>GAMAKGAVTKLKFNSPI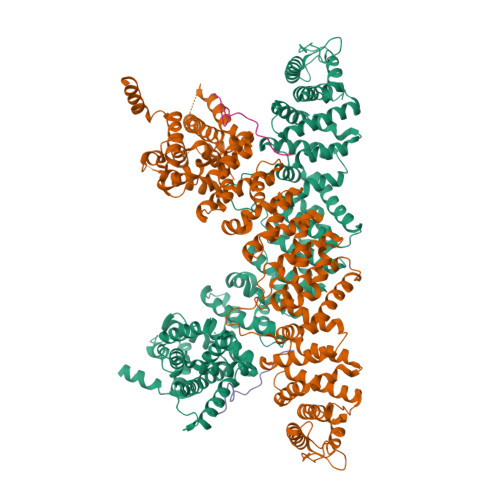ISTSDQLISTNELLDRLKALHEELASLDQDNTDLTGLDKYRDALVSRKLLKHKDVGIRAFTACCLSDILRLYAPDAPYTDAQLTDIFKLVLSQFEQLGDQENGYHIQQTYLITKLLEYRSIVLLADLPSSNNLLIELFHIFYDPNKSFPARLFNVIGGILGEVISEFDSVPLEVLRLIFNKFLTYNPNEIPEGLNVTSDCGYEVSLILCDTYSNRMSRHLTKYYSEIIHEATNDDNNSRLLTVVVKLHKLVLRLWETVPELINAVIGFIYHELSSENELFRKEATKLIGQILTSYSDLNFVSTHSDTFKAWISKIADISPDVRVEWTESIPQIIATREDISKELNQALAKTFIDSDPRVRRTSVMIFNKVPVTEIWKNITNKAIYTSLLHLAREKHKEVRELCINTMAKFYSNSLNEIERTYQNKEIWEIIDTIPSTLYNLYYINDLNINEQVDSVIFEYLLPFEPDNDKRVHRLLTVLSHFDKKAFTSFFAFNARQIKISFAISKYIDFSKFLNNQESMSSSQGPIVMNKYNQTLQWLASGLSDSTKAIDALETIKQFNDERIFYLLNACVTNDIPFLTFKNCYNELVSKLQTPGLFKKYNISTGASIMPRDIAKVIQILLFRASPIIYNVSNISVLLNLSNNSDAKQLDLKRRILDDISKVNPTLFKDQIRTLKTIIKDLDDPD[2x];>RLNTVTRVHQLMLEDAVTEREVLVTPGLEFLDDTTIPVGLMAQE[2x]>[2x]METLILTQEEVESLISMDEAMNAVEEAFRLYALGKAQMPPKVYLEFEKGDLRAMPAHLMGYAGLKWVNSHPGNPDKGLPTVMALMILNSPETGFPLAVMDATYTTSLRTGAAGGIAAKYLARKNSSVFGFIGCGTQAYFQLEALRRVFDIGEVKAYDVREKAAKKFVSYCEDRGISASVQPAEEASRCDVLVTTTPSRKPVVKAEWVEEGTHINAIGADGPGKQELDVEILKKAKIVVDDLE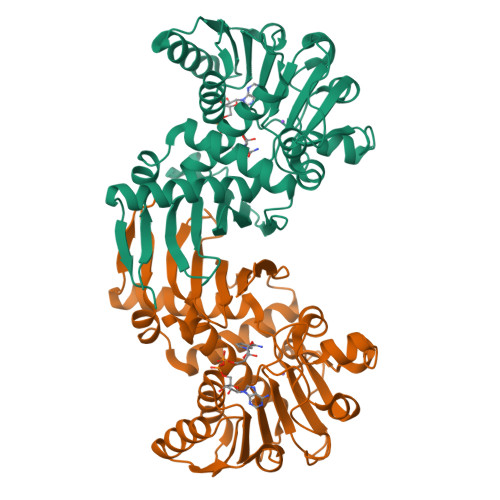QAKHGGEINVAVSKGVIGVEDVHATIGEVIAGLKDGRESDEEITIFDSTGLAIQDVAVAKVVYENALSKNVGSKIKFFRI(2S,4S)-N-((3R,5R)-1-(cyclopropanecarbonyl)-5-((3-fluoro-4-((4-(morpholinomethyl)phenyl)ethynyl)benzamido)methyl)pyrrolidin-3-yl)-4-fluoropyrrolidine-2-carboxamide 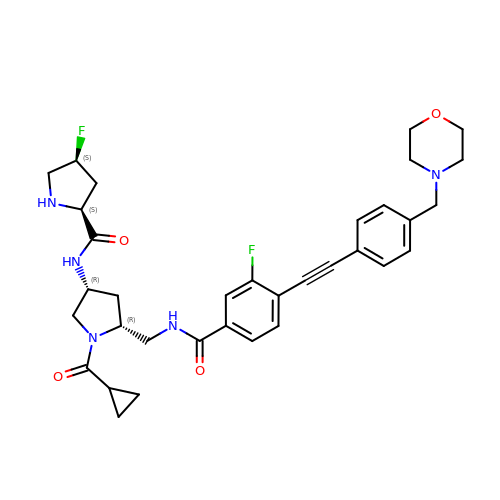| C34 H39 F2 N5 O4 | DQSZFVONXSACDZ-MLSIGSLTSA-N>MTTPISPPPQWSRRRQEKQRRLERVRGLADGAVLPREGLVAALEALIAPGDRVVLEGNNQKQADFLSRSLARVDPGKLHDLHMIMPSVGRPEHLDLFELGIARKLDFSFSGPQSLRIGQLLEDGLLEIGAIHTYIELYARLVVDLIPNVALVAGFVADREGNVYTGPSTEDTPALVEPTAFSDGIVIVQVNRIVDDPRDLPRVDIPASWVDFVVEADQPFYIEPLFTRDPRHIKPVHVLMAMMAIRGIYQRHNVQSLNHGIGFNTAAIELILPTYGESLGLKGKICRHWTLNPHPTLIPAIESGWVESVHCFGTELGMEGYIAQRPDVFFTGRDGSLRSNRMFCQLAGQYAVDLFIGATLQVDGDGHSSTVTRGRLAGFGGAPNMGHDPRGRRHSTPAWLDMRGEPEALLERGRKLVVQMVETFQDGGKPTFVERLDALEVARQTGMPLAPVMIYGDDVTHVLTEEGIAYLYKARSLEERQAMIAAVAGISPIGLRHDPRETQRMRREGLIALPEDLGIRRTDASRELLAAKSIAELVEWSGGLYQPPARFRSW[2x];>METLSFEFPAGQPGRGRALVGCVGSGDLEVLLEPGQPGKLSIQVQTSVNGSASRWQHLFERLFDGQTPPALLIDIHDFGATPGVVRLRLEQGFEEIGHD[2x];>MTDVARLLALRSFTELGARQRARALLDAGSFRELLDPFAGVQSPWLERQGIVPQADDGVVVARGLLDGQPAVLAAIEGAFQGGSLGEVSGAKIAGALELAAEDNRNGVPTRALLLLETGGVRLQEANLGLAAIAEIQAAIVDLQRYQPVVAVIAGPVGCFGGMSIAAGLCSYVLVTREARLGLNGPQVIEQEAGIAEYDSRDRPFIWSLTGGEQRFASGLADAYLADDLDEVRTSVLAYFAKGLPARPRCRRAEDYLRRLGDLDTAEQPDAAGVRRLYQGLGQGDAT[2x];>MGSSHHHHHHSQDPNSMSQPFASRGLAWFQALAGSLAPRPGDPASLRVADAELDGYPVRFLAVVPDPDNPFPRARQGEVGLLEGWGLAAAVDEALEADREAPRKRALLAIVDVPSQAYGRREEALGIHQALAGAVDAYARARLAGHPLIGLLVGKAMSGAFLAHGYQANRLIALHDPGVMVHAMGKAAAARITLRSVEELEALAAKVPPMAYDIDSYASLGLLWRTLPVETVEVPSTADLVRVRTCLGEALADILGGPRDLGGRLGAANREASARVRRLLREQW[2x]

Pseudomonas species and other aerobic bacteria have a biotin-independent malonate decarboxylase that is crucial for their utilization of malonate as the sole carbon and energy source. MdcA, MdcC, MdcD, and MdcE form the 140 kD MDC holoenzyme, with 1:1:1:1 stoichiometry among the four subunits. The malonyl-ACP is decarboxylated in the second step of the reaction to regenerate acetyl-ACP, which is catalyzed by MdcD (30 kD) and MdcE (28 kD).

By soaking crystals of the hetero-tetramer with malonyl-CoA, we obtained the structure of MDC in complex with CoA at 3.0 Å resolution (the malonate group was likely hydrolyzed during the soaking). The two hetero-tetramers in the asymmetric unit of this crystal have essentially the same conformation, with rms distance of 0.1 Å for their equivalent Cα atoms. The overall structure of this hetero-tetramer is similar to that of the malonate complex, with rms distance of ~ 0.4 Å for their equivalent Cα atoms. The electron density in the active site of MdcA is smaller than malonate in this structure, and a chloride ion is modeled in one of the active sites. We observed clear electron density for CoA, and it primarily interacts with MdcD, with its thiol group located at the center of the interface and having interactions with the main-chain amides of Val121 and Gly162 of MdcD. These two amides form the oxyanion hole for this active site, stabilizing the transition state of the decarboxylation reaction. The pyrophosphate group of CoA is located near Arg180 of MdcD, while the 3′ phosphate group of CoA is exposed to the solvent. There are substantial conformational changes for the α6–α6A segment of MdcE in the CoA complex compared to the malonate complex or the structure of MdcD–MdcE alone. In the CoA complex, helix α6 is positioned close to the adenine base of CoA. Conformational differences are also observed for the loop containing residues Val121 and Leu123, which allow these two residues to hydrogen bond and recognize the adenine base of CoA.> MTDAGRQGRVEALSISVTAPYCRFEKTGSPDLEGDETVLGLIEHGTGHTDVSLVDGAPRTAVHTTTRDDEAFTEVWHAQRPVESGMDNGIAWARTDAYLFGVVRTGESGRYADATAALYTNVFQLTRSLGYPLLARTWNYVSGINTTNADGLEVYRDFCVGRAQALDEGGIDPATMPAATGIGAHGGGITCVFLAARGGVRINIENPAVLTAHHYPTTYGPRPPVFARATWLGPPEGGRLFISATAGILGHRTVHHGDVTGQCEVALDNMARVIGAENLRRHGVQRGHVLADVDHLKVYVRRREDLDTVRRVCAARLSSTAAVALLHTDIAREDLLV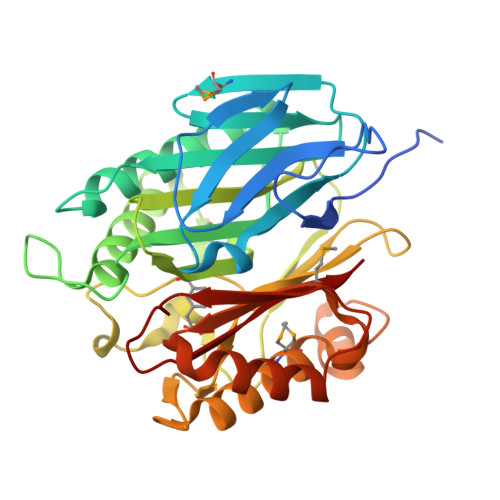EIEGMVA> LPTDTASFGRILLKKMPSVREILEERGVDMTRISAEWGEFIKKSSFTNVTSPVVLTNYLDTQYYGEIGIGTPSQTFKVIFDTGSANLWVPSTKCGPLYTACEIHNLYDSSESSSYMENGTEFTIHYGSGKVKGFLSQDVVTVGGIIVTQTFGEVTELPLIPFMLAKFDGVLGMGFPAQAVDGVIPVFDHILSQRVLKEEVFSVYYSRESHLLGGEVVLGG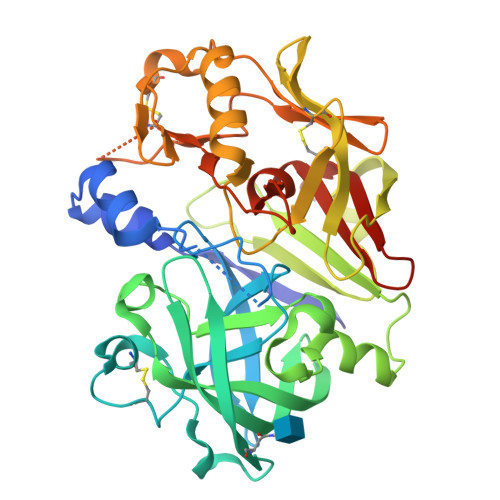SDPQHYQGNFHYVSISKAGSWQITMKGVSVGPATLLCEEGCMAVVDTGTSYISGPTSSLQLIMQALGVKEKRANNYVVNCSQVPTLPDISFYLGGRTYTLSNMDYVQKNPFRNDDLCILALQGLDIPPPTGPVWVLGATFIRKFYTEFDRHNNRIGFALARAAHHHHHH> MALENDSIAYFDGHKDSVFAIAQHPLYPNIVATGGSEGDADDAPGKGYVLDISAAAGRPVLPPSYNSDPSSAPQQNTSLNPIFEIDGHTDSINALTFTLPRGDFLVSGGMDGRMRVYAVSVPQNGALAQFKFLAESQETEEINWFAPCPSPDHPNTIALGASDGSVWVFTLDASDPSNPVQIVQSYFLHTGPCTAGAWSPDGLLLATVSEDESLHVYDVFGVAASKSLVTDNGQTVVSLTNVDQRFAVEGGLFSVAVSPTGAVVAVGGAGGQIKIVGLPRLSQPQQPQSQSQSRTGKAPAGRAGRPSQQQQTTSHQAGTILASLQIQSDNIESLAFSPSAPILAAGSTDGSIAVFDTSRSFALRRHLRGAHAEDPVVKVEFVKSPPNAAMAGWLLTSCGMDGVVRRWDLRGGTAG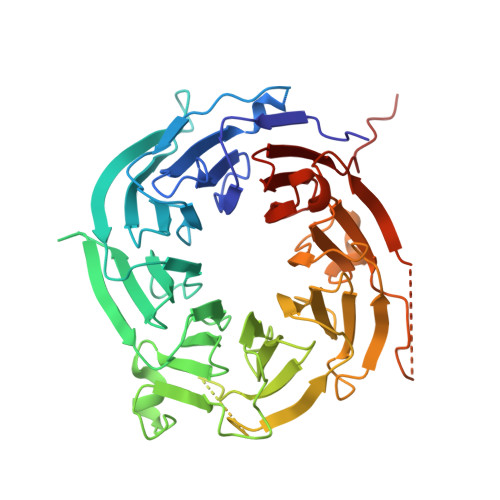PGTLPHMQHLQQQRQQQQEGAAPSGLVKEWKGHRSGQEGGGVLGFVQGETGERIVTVGDDAVVLVFEAGSHHHHHH>[2x]MNHKVHHHHHHMEETKSVQNDGAVEITSTTFESNTVAKGISNNLRIDYKILNKDKLKDGDKIVISLPDIFKDIEPKCHD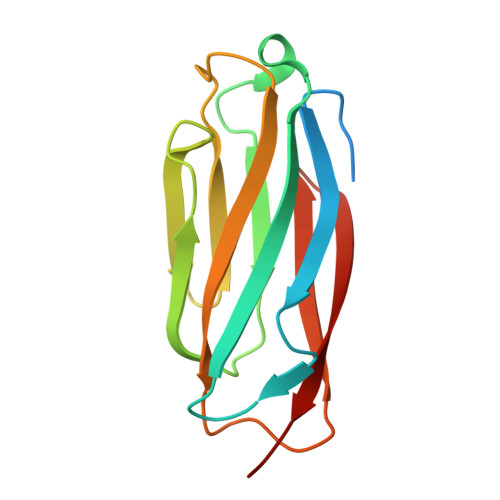QHFKDFDVKDGVVTLTFNENVEKAVTGYMIIRFVGNSNIRKGVSYPVSIDLNGKPSTVYITGEEY Here we report the discovery of type IV borosin natural product pathways (termed ‘split borosins’), featuring an iteratively acting α-N-methyltransferase and separate precursor peptide substrate from the metal-respiring bacterium Shewanella oneidensis. The α-N-methyltransferase SonM from Shewanella oneidensis MR-1 iteratively methylates its substrate SonA at two residues, SonA-L63 and SonA-I65, in an N-to-C terminal fashion on the core peptide. Complexes of SonM and SonA form dimers of heterodimers. A five helical bundle at the N-terminus of SonA, now referred to as the borosin binding domain (BBD; 1–53), serves as the SonA leader peptide and is homologous to a portion of the fused clasp region of OphMA.

The two other active site tyrosine residues, SonM-Y58 and SonM-Y71, were also mutated to phenylalanine. Both residues mainly affect the apparent kcat, where SonM-Y71F is more deleterious than SonM-Y58F (~100-fold and ~10-fold decrease in catalytic efficiency, respectively). The overall structure is very similar to wt. Loss of the hydrogen bond between the carbonyl group of “i−1” and SonM-Y58 results in minor changes, including a slight change in the interaction angle (from 108° to 114°) and a deviation from amide bond planarity (Ω angle is 178° and 174° in wt and SonM-Y58F, respectively). The core peptide of SonA-2Me is hydrogen bonded to seven SonM residues via backbone interactions. Both SonM-Y71 and SonM-Y58 are both in hydrogen bonding distance with three main chain groups of SonA-2Me. The side chain of SonM-Y58 interacts with the carbonyl and the NH groups of “i−1” (2.7 Å and 3.6 Å, respectively) and the carbonyl group of “i−3” (3.6 Å). Kinetics analysis of SonM active site mutants support a previously proposed mechanism for borosin methyltransferases, where deprotonation of the target amide nitrogen is stabilized by residues SonM-Y58, SonM-Y71, and SonM-R67.

>MGSLVCVGTGLQLAGQISVLSRSYIEHADIVFSLLPDGFSQRWLTKLNPNVINLQQFFAQNGEVKNRRDTYEQMVNAILDAVRAGKKTVCALYGHPGVFACVSHMAITRAKAEGFSAKMEPGISAEACLWADLGIDPGNSGHQSFEASQFMFFNHVPDPTTHLLLWQIAIAGEHTLTQFHTSSDRLQILVEQLNQWYPLDHEVVIYEAANLPIQAPRIERLPLANLPQAHLMPISTLLIPPAKKLEYNYAILAKLGIGPEDLG[2x];>[2x]MSGLSDFFTQLGQDAQLMEDYKQNPEAVMRAHGLTDEQINAVMTGDMEKLKTLSGDSSYQSYLVISHGNGD> SDDDWIPDIQIDPNGLSF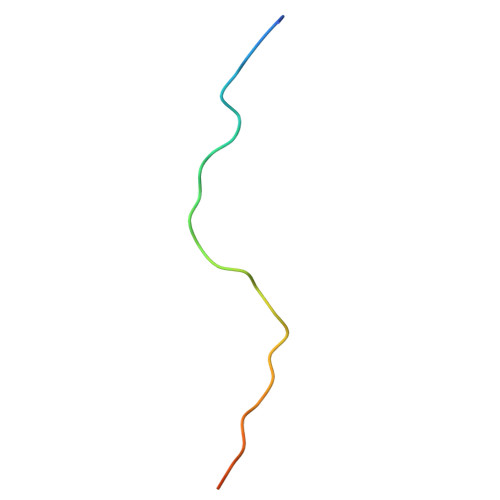NPISDFPDTTSPK> KNPHLRAYHQKIDSNLDE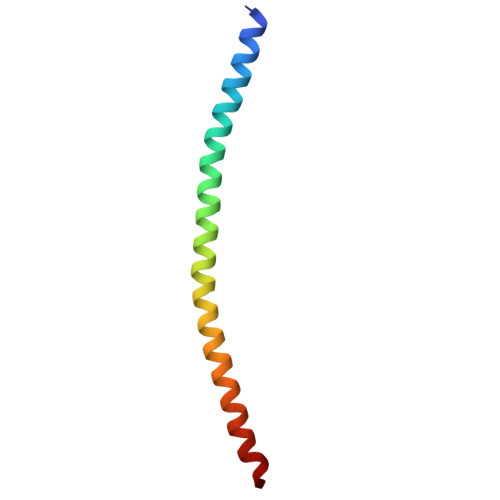LSMGLGRLKDIALGMQTEIEEQDDILDRLTTKVDKLDVNIKSTERKVRQL>[2x]DFARSLSITTPEEMIEKAKGETAYLPCKFTLSPEDQGPLDIEWLISPADNQKVDQVIILYSGDKIYDDYYPDLKGRVHFTSNDLKSGDASINVTNLQLSDIGT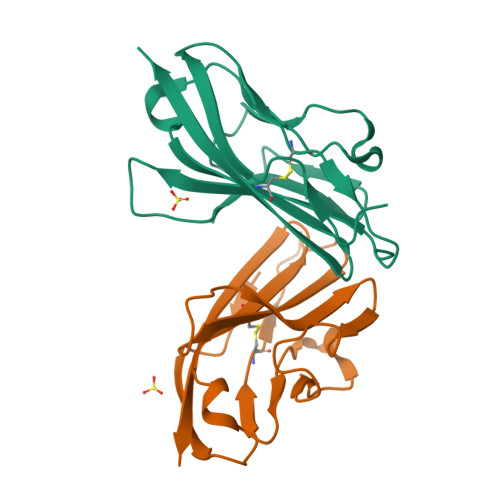YQCKVKKAPGVANKKIHLVVLVK> MTGVSDIQEAVAQIKAAGPSKPRLARDPVNQPMINNWVEAIGDRNPIYVDDAAARAAGHPGIVAPPAMIQVWTMMGLGGVRPKDDPLGPIIKLFDDAGYIGVVATNCEQTYHRYLLPGEQVSISAELGDVVGP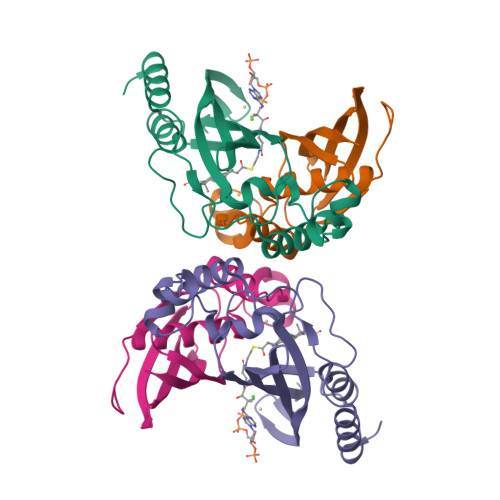KQTALGEGWFINQHIVWQVGDEDVAEMNWRILKFKPAGSPSSVPDDLDPDAMMR;> MTVVGAVLPELKLYGDPTFIVSTALATRDFQDVHHDRDKAVAQGSKDIFVNILTDTGLVQRYVTDWAGPSALIKSIGLRLGVPWYAYDTVTFSGEVTAVNDGLITVKVVGRNTLGDHVTATVELSMRDS>[2x]MEKFLVIAGPCAIESEELLLKVGEE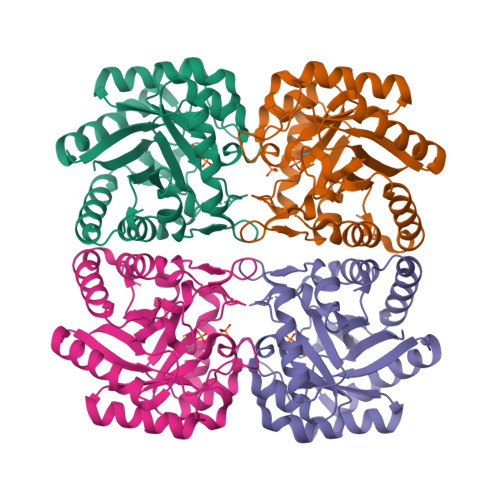IKRLSEKFKEVEFVFKSSFDKANRSSIHSFRGHGLEYGVKALRKVKEEFGLKITTDIHESWQAEPVAEVADIIQIPAFLCGQTDLLLAAAKTGRAVNVKKGQFLAPWDTKNVVEKLKFGGAKEIYLTERGTTFGYNNLVVDFRSLPIMKQWAKVIYDATHSVQLPGGLGDKSGGMREFIFPLIRAAVAVGCDGVFMETHPEPEKALSDASTQLPLSQLEGIIEAILEIREVASKYYETIPVK>MLGAVEGPRWKQAEDIRDIYDFRDVLGTGAFSEVILAEDKRTQKLVAIKCIAKEALEGKEGSMENEIAVLHKIKHPNIVALDDIYESGGHLYLIMQLVSGGELFDRIVEKGFYTERDASRLIFQVLDAVKYLHDLGIVHRDLKPENLLYYSLDEDSKIMISDFGLSKMEDPGSVLSTACGTPGYVAPEVLAQKPYSKAVDCWSIGVIAYILLCGYPPFYDENDAKLFEQILKAEYEFDSPYWDDISDSAKDFIRHLMEKDPEKRFTCEQALQHPWIAGDTALDKNIHQSVSEQIKKNFAKSKWKQAFNATAVVRHMRKLQ[2x]

When activated, CaM binds to and stimulates the activities of a family of Ca2+/CaM-dependent serine/threonine protein kinases (CaMKs), thereby regulating their functions. However, the regulation mechanism of CaMKI remains elusive. Here we report four crystal structures of three truncation variants of human CaMKIα, namely CaMKI320 (residues 1–320), CaMKI315 (residues 1–315), and CaMKI293 (residues 1–293), which correspond to the aforementioned three truncation forms of CaMKI, respectively. The catalytic core of CaMKI takes a canonical bilobate architecture, with the N-terminal lobe (N lobe) consisting of five antiparallel β-strands and a prominent helix named helix αC and the C-terminal lobe (C lobe) comprised primarily of α-helices.

Therefore, we co-crystallized CaMKI320 with ATP and successfully obtained the complex structure, in which ATP is observed with evident electron density; however, no Mg2+ was visible despite the presence of 20 mM MgCl2 in the protein solution. Upon ATP binding, CaMKI320 undergoes significant conformational changes characterized by a different N lobe orientation, the disordering of helix αT of the activation segment, and the formation of helix αR2 of the CaM-binding segment compared with the apo CaMKI320. In particular, the residues on strand β1 of the P-loop exhibit positional displacements of about 5–7 Å, and ATP bound at the nucleotide-binding site interacts with the surrounding residues via a network of hydrogen bonds. The CaMKI320-ATP complex displays structural features of an inactive conformation. Compared with the apo CaMKI320, although the structure elements forming the nucleotide-binding site show significant positional displacements up to 7 Å and helix αC is rotated towards strands β3-β5, Glu66 and Lys49 does not form a salt bridge which is critical for the maintenance of the active kinase. Intriguingly, in the CaMKI320-ATP complex, the CaM-binding segment mainly forms a long αR2 helix which protrudes away from the catalytic core. A detailed analysis indicates that helix αR2 of this conformation plays an important role in the maintenance of an inactive state of the enzyme through interaction with Glu102 and stabilization of the inactive conformations of helices αR1 and αD. Specifically, Lys300 on helix αR2 also forms a salt bridge with Glu102; this interaction does not abrogate the ability of Glu102 to bind ATP as Glu102 still makes hydrogen-binding interactions with the 2′- and 3′-hydroxyls of the ribose moiety of ATP, however, it could have an impact on its ability to bind the substrate as Glu102 is also suggested to play a role in the recognition and binding of Arg at P(-3) of the substrate (see discussion above). Furthermore, the side chain of Gln305 of αR2 forms two hydrogen-bonding interactions with the side chains of Ser291 and Lys295, and thus helix αR2 also contributes to stabilization of helix αR1 in the inactive conformation.>[24x]TGWSHPQFEKLKGGS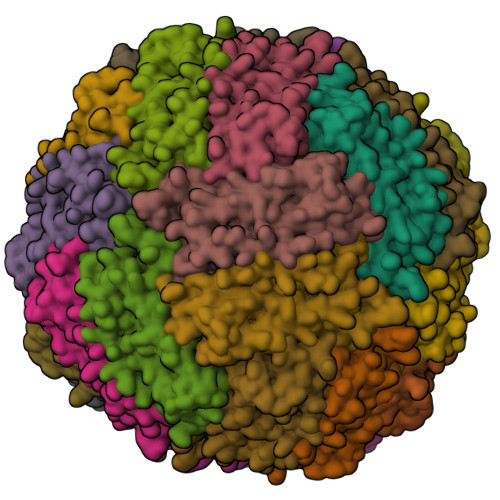SRGGGGGSGGSGGSGGSMSSQIRQNYSTDVEAAVNSLVNLYLQASYTYLSLGFYFDRDDVALEGVSHFFRELAEEKREGYERLLKMQNQRGGRALFQDIKKPAEDEWGKTPDAMKAAMALEKKLNQALLDLHALGSARTDPHLCDFLETHFLDEEVKLIKKMGDHLTNLHRLGGPEAGLGEYLFERLTLRHDGGSGGSGGSGGSGGGASGGS> CTNEDGKP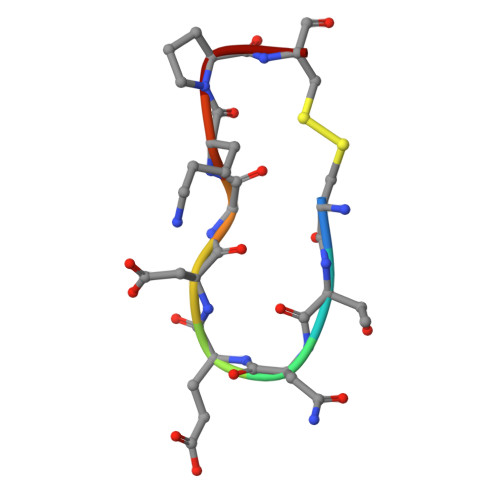C>MGFAVESRSHVKDILGLINTFNEVKKITVDGTTPITVAHVAALARRHDVKVALEAEQCRARVETCSSWVQRKAEDGADIYGVTTGFGACSSRRTNQLSELQESLIRCLLAGVFTKGCASSVDELPATVTRSAMLLRLNSFTYGCSGIRWEVMEALEKLLNSNVSPKVPLRGSVSASGDLIPLAYIAGLLIGKPSVIARIGDDVEVPAPEALSRVGLRPFKLQAKEGLALVNGTSFATALASTVMYDANVLLLLVETLCGMFCEVIFGREEFAHPLIHKVKPHPGQIESAELLEWLLRSSPFQDLSREYYSIDKLKKPKQDRYALRSSPQWLAPLVQTIRDATTTVETEVNSANDNPIIDHANDRALHGANFQGSAVGFYMDYVRIAVAGLGKLLFAQFTELMIEYYSNGLPGNLSLGPDLSVDYGLKGLDIAMAAYSSELQYLANPVTTHVHSAEQHNQDINSLALISARKTDEALDILKLMIASHLTAMCQAVDLRQLEEALVKVVENVVSTLADECGLPNDTKARLLYVAKAVPVYTYLESPCDPTLPLLLGLKQSCFGSILALHKKDGIETDTLVDRLAEFEKRLSDRLENEMTAVRVLYEKKGHKTADNNDALVRIQGSRFLPFYRFVRDELDTGVMSARREQTPQEDVQKVFDAIADGRITVPLLHCLQGF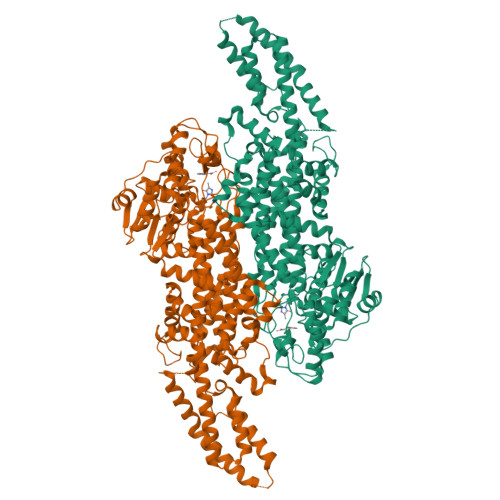LGQPNGCANGVESFQSVWNKSA[2x]>ANKPMQPITSTANKIVWSDPTRLSTTFSASLLRQRVKVGIAELNNVSGQYVSVYKR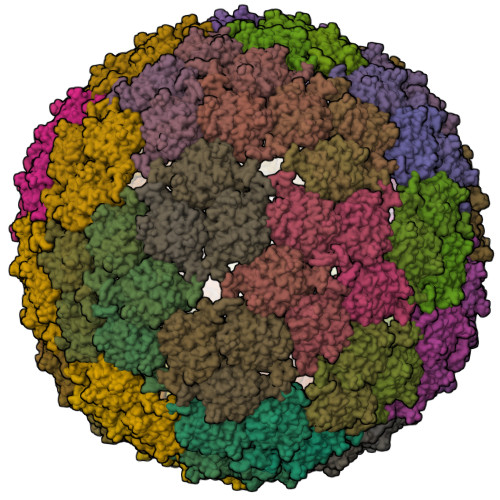PAPKPEGCADACVIMPNENQSIRTVISGSAENLATLKAEWETHKRNVDTLFASGNAGLGFLDPTAAIVSSDTT[240x]N-{[3-(biphenyl-4-yl)propanoyl]carbamoyl}-beta-D-glucopyranosylamine 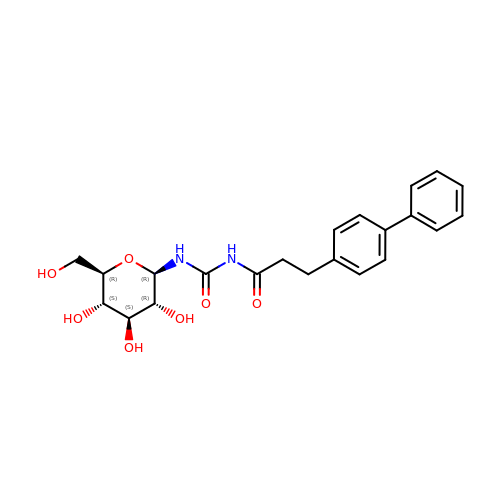| C22 H26 N2 O7 | DTCZORBBXRCGBE-QNDFHXLGSA-N TRIFLUOROACETONYL 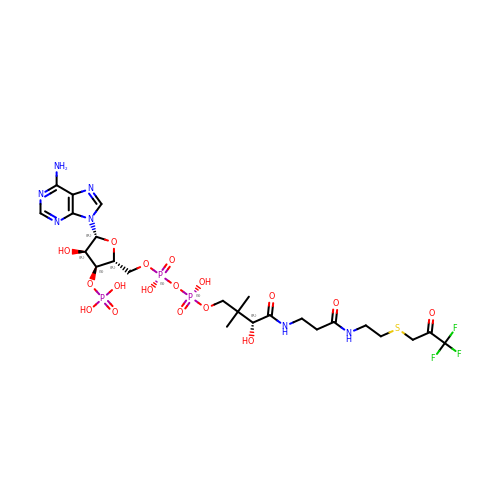COENZYME A | C24 H37 F3 N7 O17 P3 S | XDIQTPZOIIYCTR-GRFIIANRSA-N>SQQLQKEEEARKVKSGIRQMRLFSQDECAKIEARIDEVVSRAEKGLYNEHTVDRAPLRNKYFFGEGYTYGAQLQKRGPGQERLYPPGDVDEIP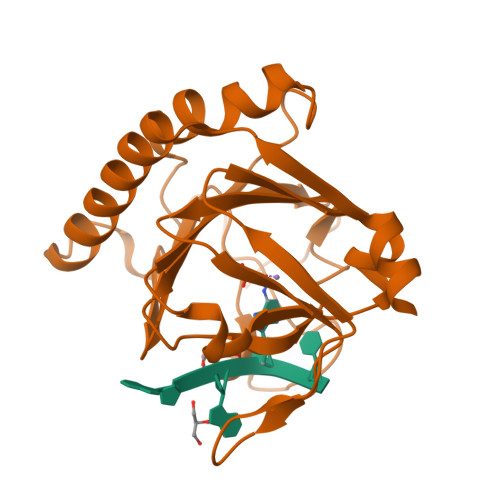EWVHQLVIQKLVEHRVIPEGFVNSAVINDYQPGGCIVSHVDPIHIFERPIVSVSFFSDSALCFGCKFQFKPIRVSEPVLSLPVRRGSVTVLSGYAADEITHCIRPQDIKERRAVIILRKTRLDAPRL[3x]To further explore this issue, we have conducted biochemical and crystallographic studies on the interactions of six GSTOs from T. versicolor with chemical libraries. The six TvGSTOs (named TvGSTO1S to TvGSTO6S) used in this study are representatives of the twelve TvGSTOs that have a catalytic serine, while four others have a cysteine instead. In this study, we demonstrated at the biochemical and structural level that T. versicolor GSTs that belong to the Omega class interact with polyphenolic compounds found in wood, and in particular with flavonoids such as dihydrowogonin and naringenin. The ability of TvGSTOs to bind polyphenols through different sites suggests that fungal GSTs could be involved in the transport of various polyphenols.

Indeed, a few compounds significantly increased the stability of TvGSTO1S, 3S and 6S, i.e. they show a variation of the denaturation temperature ∆Td > 5 °C. On the contrary, most chemical compounds induced a destabilizing effect on TvGSTO5S and 2S (∆Td < 0 °C), whereas the chemical library had little impact on TvGSTO4S thermal stability. As shown with TSA, other TvGSTO isoforms also interact with HBPs, each with its own selectivity. The alignment of the solved structures with the sequences of TvGSTO1S, −2S, −4S and −5S shows variations at the putative H- and L-sites, which could explain the isoform-specific TSA patterns.

>[2x]MPCTEQITLYTTTFSPYGHRAHIALEEAGAEYTLCQINVHRDKPEWYKRVNPLGKVPAITFGGPQVPPDEPSPESEKLVESLALLEFVADVFPEAKLLPASPVQRARARAFIAIYQNYLHDQFRDAFFRGEPVGPFLQALETLQSALPPAGFAVGEWSLAEAAVAPFLARMMLYLDAGLGKYSEADGETMRAALASERFARISQYVRDIRARASFVKSWGGDDVQLEAAKAIPMLRRPAHHHHHH>[3x]MATFVRNAWYVAALPEELSEKPLGRTILDTPLALYRQPDGVVAALLDICPHRFAPLSDGILVNGHLQCPYHGLEFDGGGQCVHNPHGNGARPASLNVRSFPVVERDALIWIWPGDPALADPGAIPDFGCRVDPAYRTVGGYGHVDCNYKLLVDNLMDLGHAQYVHRANAQ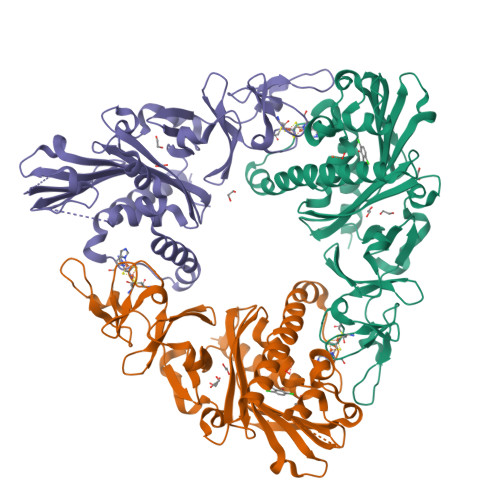TDAFDRLEREVIVGDGEIQALMKIPGGTPSVLMAKFLRGANTPVDAWNDIRWNKVSAMLNFIAVAPEGTPKEQSIHSRGTHILTPETEASCHYFFGSSRNFGIDDPEMDGVLRSWQAQALVKEDKVVVEAIERRRAYVEANGIRPAMLSCDEAAVRVSREIEKLEQLEAARLEHHHHHH> GSHMLFAEFAEFCERLEKISSTLELTARIAAFLQKIEDERDLYDVVLFITGKVYPPWDERELGVGIGLLYEALENVSGVKRSEIESMIREYGDLGLVAEQLIKKKKMTTLAFEELTVRKVRETFDEIASLTGEGSMKRKIMLLTGLYGLATPLEARYLTRLILNEMRLGVGEGIMRDAIARAFRADPETVERAYMITNDLGRVAVVAKKEGEEGLRKMKIEIHIPVRMMLAQVAESLESAVREMRTAAVEWKFDGSR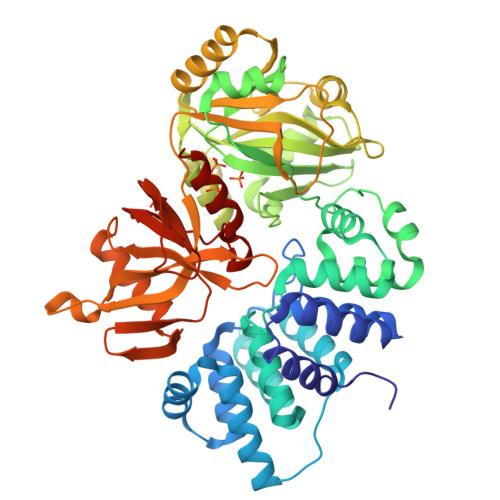VQVHWDGSRVTIYSRRLENVTNALPDIVEEIKKSVKPGVILDGEVIAVKEGKPMPFQHVLRRFRRKHDVAKMVEKIPLEAHFFDILYHDGECIDLPLRERRKLLESAVNESEKIKLAKQIVTDSVDEVRKMYDEAISAGHEGVMIKLPSSPYIPGKRGKNWLKVKAIMETLDLVVVGGEWGEGKRSHWLSSFELACLDPVTGKLLKVGRVATGFTEEDLEELTEMFRPLIVSQQGKKVEFIPKYVFEVAYQEIQKSPKYESGYALRFPRFVRLRDDKDVDEADTIERVENLYKLQFEVKRQ>GGKNTETAAKKEYKPSAMEQMNAKNDPNVIQDNYRTCYEVFVYSFFDSDGDGIGDLKGLTEKLDYIEGLGCNEIWMMPI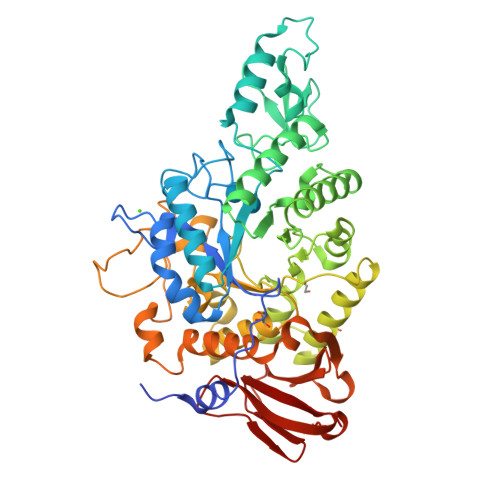MPSPSYHKYDITDYMNIDKQYGTLDDFDALITECHKRNINVIIDFVINHTSNEHPWFKAAADYIKSLPDGAEPDSSECPYVDYYNFSKTNTGGYNQLPGTNWYYESQFVDSMPDLNLQSEAVRGEIDKVTSFWLDRGVDGFRLAAVIYYNNNNQTETIDDLTWLVNNVKSKKADAYMVGEGWTTYREYAKYYKSGIDSMFNFDFSQQDGYIGKVLNGAANHGASTYGNALVDVENEIKKYTDSYIDAPFYTNHDMGRSAGYYNGDNAEEKTKMAQAMNLLMPGNAFLYYGEEIGMRGTANDETKRLAMRWSGDSKAKGMCVGPQNAEETEQTYDTLDKQMEDPYSIYNFVKQTISIRNAFPEIARGTNTFEKDLSNDNVCIFTREYNGEKAVLIFNPSKDEASVDVSSLGVNDAVAMLQTTAAAPSYKDGTAKLPAYSVLVLKENLY[2x]> MPRLSLRIVLCLATALSTLPVHAESRDDAAEVAPSTRPEPSLEQAFKDPPSSARPRVWWHWMNGNITKDGIRKDLEWMKRVGIGGLQNFDANLQTPQIVDHRLVYMTPEWKDAFRFAAHEADRLDLELAIAASPGWSETGGPWVKPQDGLKKLVWSETTLAGGQRFVGRLASPPGTTGPFQTLHPPVTIEEIISGVPAETGGVSYAGEVGVLAFPVPDIASLPVPRALDGAGNVLAGKALVDADIAGGVTLARVDGKAPLLRLDYQRPVTVRSATVFVPNVRIPFAGAAFAGTLESSQDGKTWTPIKALELSNVPTTISFAPVEAAHFRLVLNPGQPDAALGSPAPGVAGNDLFGAIASKRAGQPIMVGQFELHSDALVDRYETKAGFVMSRDYYALVGPHDNVTGVDPDSVIDLTDKLKADGTLDWAAPKLPAGQHWRVLRLGYSLLGTTNHPAPPEATGLEVDKFDGEAVREYLEHYIGMYKDAAGPDMVGKRGVRALLTDSIEVGEANWTPRMLEQFQRLRGYDARPWLPALTGTLVGTREQSDRFLYDYRRTLADLLASEHYGTVADVAHENDLKVYGEALEDHRPMLGDDMAMRSHADIPMAALWTFNRDEGPRQTLIADMKGAASVAHLYGQNLVAAESMTASMAPWAFAPKDLKRFIDLEFVTGVNRPVIHTSVHVPVDDKKPG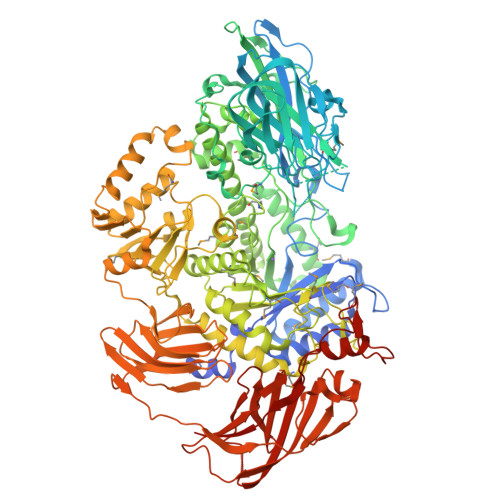LSLAIFGQYFNRQESWAEMARPWVDYIARSSLLLQTGRNVADVAYFYGEEAPLTGLYGDEPVADAPVRYAYDYINFNALTELLANDGEDLVAPSGARYKTIYLGGSSSHMTLAALRKLAALVVGGATVVGKAPIATPSNTSAQEGDLTEWSSLVARLWPGSGDARVGKGRVIASQDIESALQAMDVAPDFTFTGADAGVKIPFVHRRDGKGEIYYLVNQQEAAQSIEAHFRVTGKQPELWHPETGKSEPISYRISGGETVVPLHLDGDEAVFVVFRKAAARDRVTLARQGERAVATLDGAWQVAFQADRGAPASIELARLEPLDKSADPGVKYFSGIATYSRNFRVTGKYGEGRSLWLDLGRVGDLAQVSVNGVDVGTAWHAPYRLDIGKAVRKGQNTLEIRVANTWVNRLIGDQQEGAQKITWTAMPTYRADAPLRPSGLIGPVRLIEETTGGHHHHHH> MTALTESSTSKFVKINEKGFSDFNIHYNEAGNGETVIMLHGGGPGAGGWSNYYRNVGPFVDAGYRVILKDSPGFNKSDAVVMDEQRGLVNARAVKGLMDALDIDRAHLVGNAMGGATALNFALEYPDRIGKLILMGPGGLGPSMFAPMPMEGIKLLFKLYAEPSY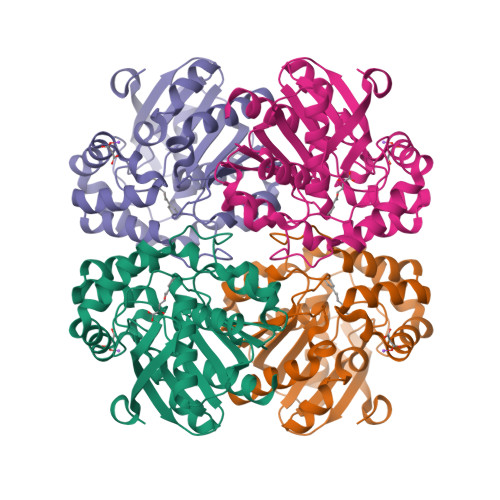ETLKQMLQVFLYDQSLITEELLQGRWEAIQRQPEHLKNFLISAQKAPLSTWDVTARLGEIKAKTFITWGRDDRFVPLDHGLKLLWNIDDARLHVFSKCGHWAQWEHADEFNRLVIDFLRHA> MQAIKESYAFAVLGEPRYAFNFNHFDYVNPAAPKGGQITLSALGTFDNFNRYALRGNPGARTEQLYDTLFTTSDDEPGSYYPLIAESARYADDYSWVEVAINPRARFHDGSPITARDVEFTFQKFMTEGVPQFRLVYKGTTVKAIAPLTVRIELAKPGKEDMLSLFSLPVFPEKYWKDHKLSDPLATPPLASGPYRVTSWKMGQNIVYSR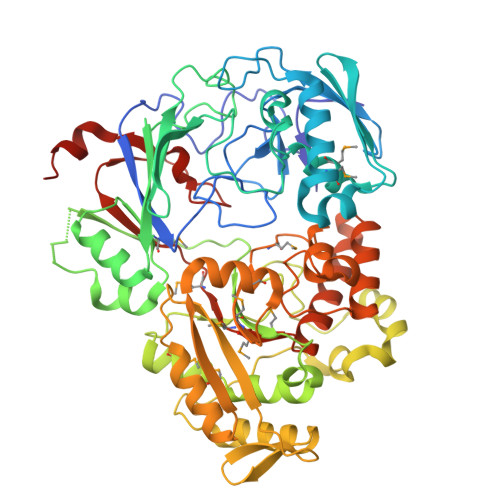VKDYWAANLPVNRGRWNFDTIRYDYYLDDNVAFEAFKAGAFDLRMENDAKNWATRYTGKNFDKKYIIKDEQKNESAQDTRWLAFNIQRPVFSDRRVREAITLAFDFEWMNKALFYNAWSRTNSYFQNTEYAARNYPDAAELVLLAPMKKDLPSEVFTQIYQPPVSKGDGYDRDNLLKADKLLNEAGWVLKGQQRVNATTGQPLSFELLLPASSNSQWVLPFQHSLQRLGINMDIRKVDNSQITNRMRSRDYDMMPRVWRAMPWPSSDLQIAWSSEYINSTYNAPGVQSPVIDSLINQIIAAQGNKEKLLPLGRALDRVLTWNYYMLPMWYMAEDRLAWWDKFSQPAVRPIYSLGIDTWWYDVNKAAKLPSASKQGE> MITITTIFVPRDSTALALGADDVARAIAREAAARNEHVRIVRNGSRGMFWLEPLVEVQTGAGRVAYGPVSAADVPGLFDAGLLQGGEHALSQGVTEEIPFLKQQERLTFARVGITDPLSLDDYRAHEGFAGLERALAMQPAEIVQEVTDSGLRGRGGAAFPTGIKWKTVLGAQSAVKYIVCNADEGDSGTFSDRMVMEDDPFMLIEGMTIAALAVGAEQGYIYCRSEYPHAIAVLESAIGIANAAGWLGDDIRGSGKRFHLEVRKGAGAYVCGEETALLESLEGRRGVVRAKPPLPALQGLFGKPTVINNVISLATVPVILARGAQYYRDYGMGRSRGTLPFQLAGNIKQGGLVEKAFGVTLRELLVDYGGGTRSGRAIRAVQVGGPLGAYLPESRFDVPLDYEAYAAFGGVVGHGGIVVFDETVDMAKQARYAMEFCAIESCGKCTPCRIGST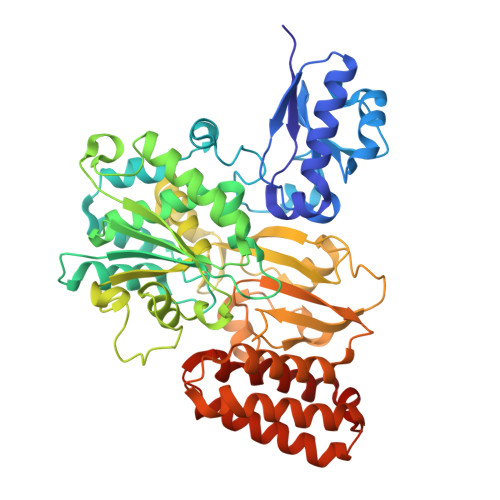RGVEVMDRIIAGEQPVKHVALVRDLCDTMLNGSLCAMGGMTPYPVLSALNEFPEDFGLASNPAKAA>[3x]GSAMARTEKIYIYGASGHGLVCEDVAK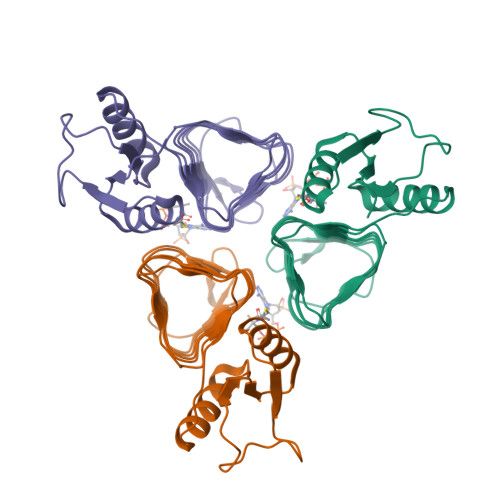NMGYKECIFLDDFKGMKFESTLPKYDFFIAIGNNEIRKKIYQKISENGFKIVNLIHKSALISPSAIVEENAGILIMPYVVINAKAKIEKGVILNTSSVIEHECVIGEFSHVSVGAKCAGNVKIGKNCFLGINSCVLPNLSLADDSILGGGATLVKNQDEKGVFVGVPAKRM>[10x]EERLHYQVGQRALIQAMQIS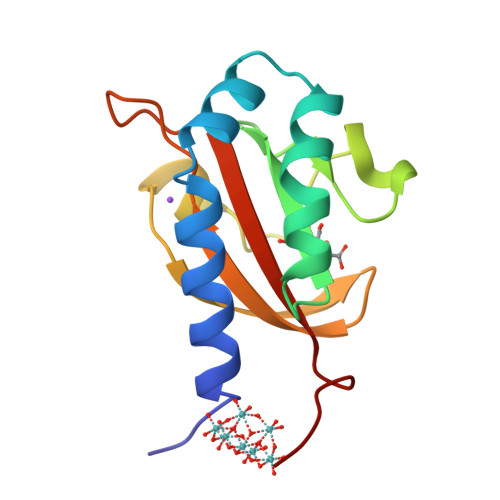AMPELVEAVQKRDLARIKALIDPMRSFSDATYITVGDASGQRLYHVNPDEIGKSMEGGDSDEALINAKSYVSVRKGSLGSSLRGKSPIQDATGKVIGIVSVGYTIEQLEHH> MKKHHHHHH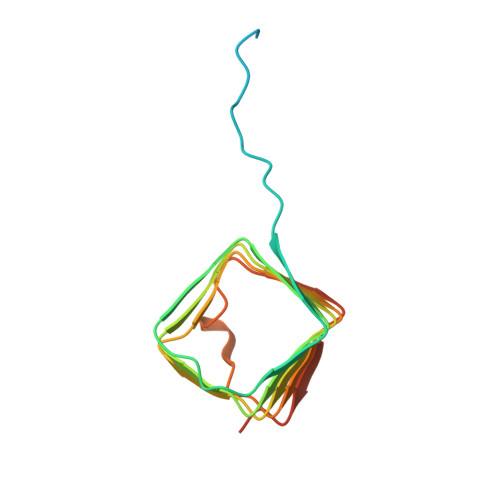GSLVPRGSDVIKPLQSDEYALLTRNVERDKYANFTINFTMENQIHTGMEYDNGRFIGVKFKSVTFKDSVFKSCTFEDVTSVNTYFKNCTFIDTVFDNTDFEPYKFIDSEFKNCSFFHNKTGCQITFD> SNAMANYLVTGGSKGIGKAVVELLLQNKNHTVINIDIQQSFSAENLKFIKADLTKQQDITNVLDIIKNVSFDGIFLNAGILIKGSIFDIDIESIKKVLDLNVWSSIYFIKGLENNLKVGASIVFNGSDQCFIAKPNSFAYTLSKGAIAQ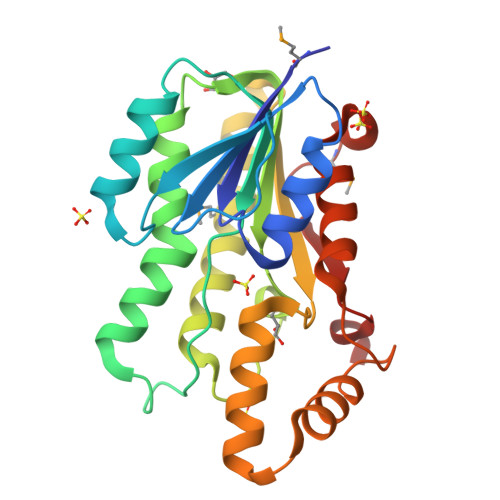MTKSLALDLAKYQIRVNTVCPGTVDTDLYRNLIQKYANNVGISFDEAQKQEEKEFPLNRIAQPQEIAELVIFLLSDKSKFMTGGLIPIDGGYTAQ>[2x]HHHHH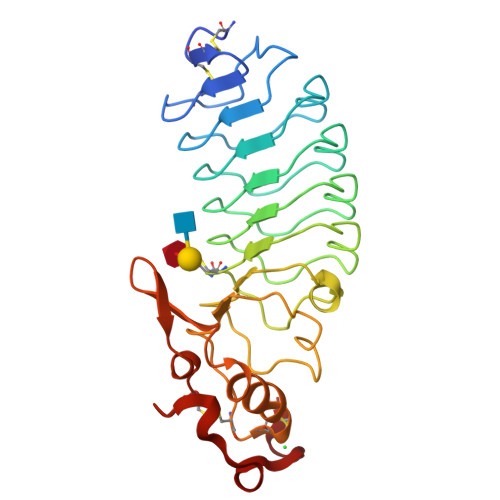HCPSQCSCSGTTVNCKSKSLASVPAGIPTTTRVLYLNDNQITKLEPGVFDRLVNLQTLWLNNNQLTSLPAGLFDSLTQLTILALDSNQLQALPVGVFGRLVDLQQLYLGSNQLSALPSAVFDRLVHLKELLMCCNKLTELPRGIERLTHLTHLALDQNQLKSIPHGAFDRLSSLTHAYLFGNPWDCECRDIMYLRNWVADHTSIVMRWDGKAVNDPDSAKCAGTNTPVRAVTEASTSPSKCP> ARLGARPCGLRELEVRVSELGLG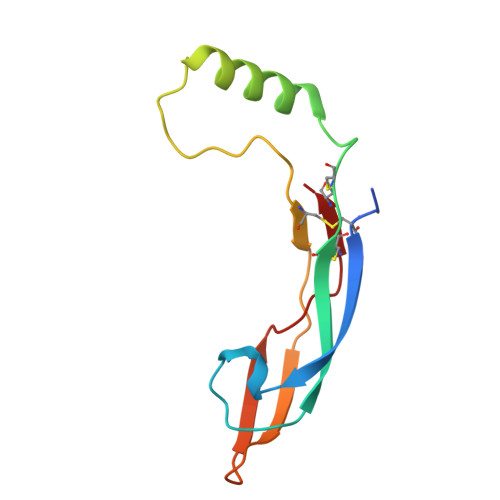YASDETVLFRYCAGACEAAARVYDLGLRRLRQRRRLRRERVRAQPCCRPTAYEDEVSFLDAHSRYHTVHELSARECACV> MGSHHHHHHSSGLVPRGSHMFKREEIIEMANKDFEKAWIETKDLIKAKKINESYPRIKPVFGKTHPVNDTIENLRQAYLRMGFEEYINPVIVDERDIYKQFGPEAMAVLDRCFYLAGLPRPDVGLSDEKISQIEKLGIKVSEHKESLQKILHGYKKGTLDGDDLVLEISNALEISSEMGLKILEDVFPEFKDLTAVSSKLTLRSHMTSGWFLTVSDLMNKKPLPFKLFSIDRCFRREQKEDKSHLMTYHSASCAIAGEGVDINDGKAIAEGLLSQFGFTNFKFIPDEKKSKYYTPETQTEVYAYHPKLKEWLEVATFGVYSPVALSKYGIDVPVMNLGLGVERLAMISGNFADVREMVYPQFYEHKLNDRNVASMVKLDKVPVMDEIYDLTKELIESCVKNKDLKSPCELAIEKTFSFGKTKKNVKINIFEKEEGKNLLGPSILNEIYVYDGNVIGIPESFDGVKEEFKDFLEKGKSEGVATGIRYIDALCFKITSKLEEAFVSNTTEFKVKVPIVRSLSDINLKIDDIALKQIMSKNKVIDVRGPVFLNVEVKIEXXXXXX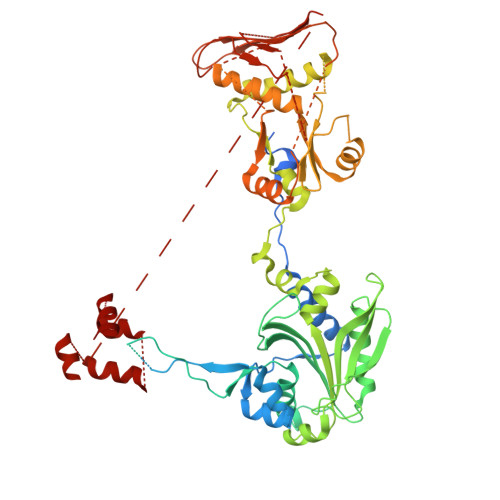XXXXXXXXXXXXXXXXXXXXXXXXXXXXXXXXXXXXXXXXXXXXXXXXXXXXXXXXXXXXXXXXXXXXXXXXXXXXXXXXXXXXXX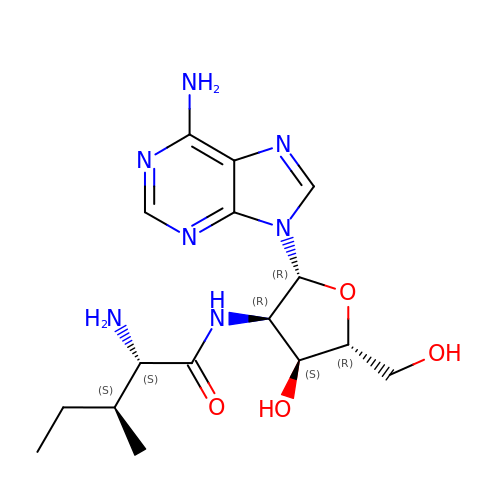2'-(L-ISOLEUCYL)AMINO-2'-DEOXYADENOSINE | C16 H25 N7 O4 | GWYBWPBDPROZEC-DTKXOMKJSA-N> CGCGXAUUAGCG

When deamination affects guanosines, a xanthosine (X) containing RNA is generated. Applying NMR spectroscopy and X-ray crystallography, we demonstrate that X can form distinct wobble geometries with uridine depending on the sequence context. In contrast, X pairing with cytidine occurs either through wobble geometry involving protonated C or in Watson–Crick-like arrangement. We therefore utilized the 27 nt fragment of the E. coli 23S rRNA sarcin−ricin loop (SRL), the 12 nt RNA 5′-CGCGAAUUACGC, and the 14 nt RNA 5′-GGUAUUGCGGUACC, all of them are known crystallization scaffolds.

Therefore, we switched to a different crystallization scaffold, namely 5′-CGCGAAUUACGC, and fortunately, we obtained another structure of a X–U modified RNA at high resolution. Replacement of A5 by X5 gave crystals that diffracted at 1.0 Å resolution. Surprisingly, the X5–U8′ base pair adopted a wobble conformation (w2U–X) distinct to a typical G–U pair, involving X-N1H•••O4-U and X-O2•••HN3-U hydrogen bonds. A possible rationale for this alternative wobble geometry is that the neighboring base pair is not a standard Watson–Crick pair but a purine-purine pair (G4-A9) that widens the helix. This specific environment likely renders the w2U–X geometry energetically favorable. Interestingly, the X5-U8′ base pair coordinates a metal ion which is assigned to sodium based on the coordination geometry and the distances of 2.4 to 2.5 Å to the six coordination sites. These are O6 of X5, O4 of U8′, and the O4 atom of U7′ with the remaining sites of the ion occupied by water molecules. Of note, both the riboses of xanthosine and the paired uridine are in C3′-endo conformation. Analysis of the 5′-CGCGXAUUACGC by 1H-NMR spectroscopy indicated that the system is rather dynamic in solution likely existing in equilibrium between hairpin and duplex conformations. In particular, for the 12 and 14 nt RNAs, solution NMR spectroscopy indicated structural dynamics that we could not resolve further with standard NMR experiments applied.>MHHHHHHDREMLEGYLKDRLGKVLEIYPASVKRKEDAIFFMVKNREDGEKYLVVIGSADVTEEFSGDYVGEIALEKSKAKSKVKISERNHNNLLVLRQYLPWLNPSVCGKRSSFGTGDRLGIATPAHVKAFEGKECFPFLAQQSVREMSRTGRNWLSVLDDAIWGIFESGYEGAFGADADHVKDLEDIKTAIDAGYTMFTIDPSDHVLDPSTIDKAAAEHVFFELNERHDFLSKYEEKVYEIGGRKYTFDRDSLIETVITYGKAVDHVEKCYLFLKENNRNPFELEVSVDETSTPTTPLAHIFIVEELKRRGVVFTNLALRFVGEWQKAIDYIGDLKELDSTLAEHAAIAEVLGPYKLSLHSGSDKFSAYPYFAKHVGNLFHVKTAGTSYLEAIRVVARFSPELYRRIHEFALQRFEKDRASYHVTTDLSKVPDISKIPDSQLEDLLNEPNTRQVIHITYGSVLTARNSDGSYLFRDELFKTLSEHEREHYEQVASH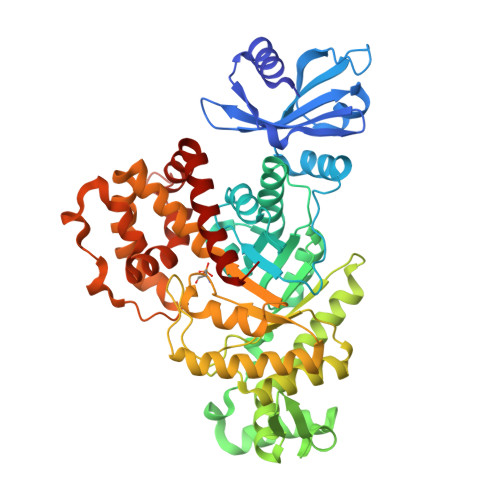IRKHLDLLGV[5x]> GSHMQKDFWLSEIGDKNISLGYYDDNVAIVLTNKTDKILRVYSYEDGKIRKDFEQKEIITGLMGDKKIEGDLKTPVGFYELGRKFNPGDPYYGPFAFATTYPNLLDKVQGKTGGGIWIHGYPLDGSRLDEFKTRGCIALFNNNLEKFAQVVQDKKVFVMTEEKEKIRAKKDQIASLLADLFTWKLAWTNSDTNTYLSFYDEQEFKRFDKMKFEQFASMKKSIFSRKEDKKIKFSDINISPYPNLENETMYRISFY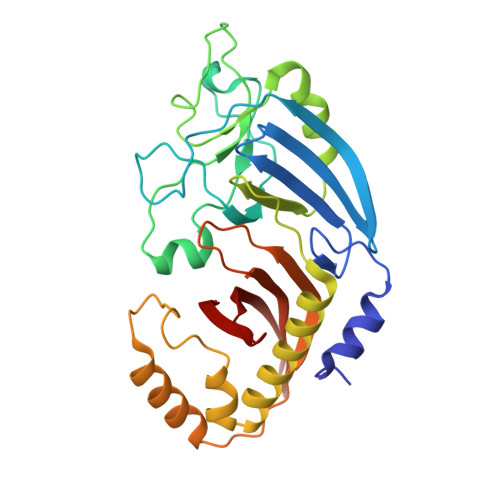EDYYTKNYQFRGDKILYVKIDSKGKMKILAEQ>MASWSHPQFEKSGGGGGLVPRGSQVFLEERLDGATGSSIVVTMEGTRPILAEVQALVTPTMFGNAKRTTTGLDFNRASLIMAVLEKRAGLLLQNQDAYLKSAGGVKLDEPAIDLAVAVAIASSYKDKPTNPQECFVGELGLTGEIRRVNRIEQRINEAAKLGFTKI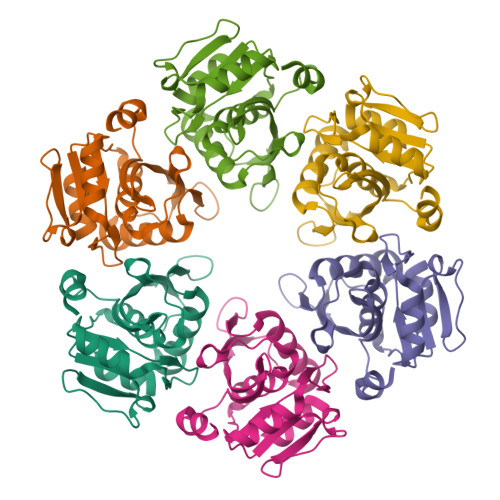YVPKNSLTGITLPKEIQVIGVTTIQEVLKKVF[2x]>[2x]SNELKVREFYRLHNACVKLKESIKLIYENPLVTDQNVLNLGTAEN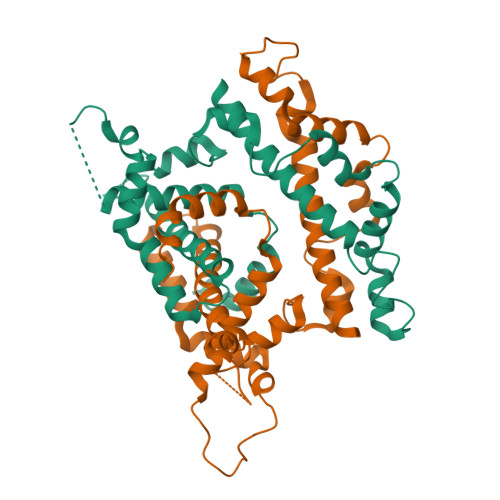TIDYTILNTPTLNVAKTLLGNRYSLDLIDLFQSHDFKDSNTDVDMFIKYPVVYDENLENLAFMHKSFPNMNAHLNDAQKTQLSNERLEFLGDSWLGALVSYIVYTRFPSANEGMLSQMKESIVNNNNLFDWSTKLNFTKRLQGNIATPTRVVKDKMSKRYADCVQAYIGALVIDRFGTEFLDIKEWLEELSEKKLAKSSQM NITROFURAZONE | C6 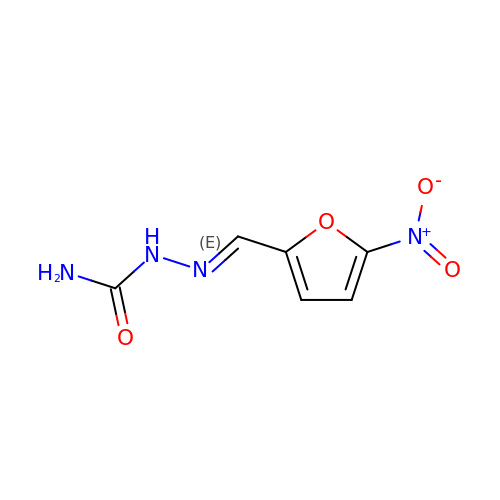H6 N4 O4 | IAIWVQXQOWNYOU-FPYGCLRLSA-N>MAEKPKLHYFNARGRMESTRWLLAAAGVEFEEKFIKSAEDLDKLRNDGYLMFQQVPMVEIDGMKLVQTRAILNYIASKYNLYGKDIKERALIDMYIEGIADLGEMILLLPVCPPEEKDAKLALIKEKIKNRYFPAFEKVLHHHGQDYLVGNKLSRADIHLVELLYYVEELDSSLISSFPLLKALKTRISNLPTVKKFLQPGSPRKPPMDEKSLEEAR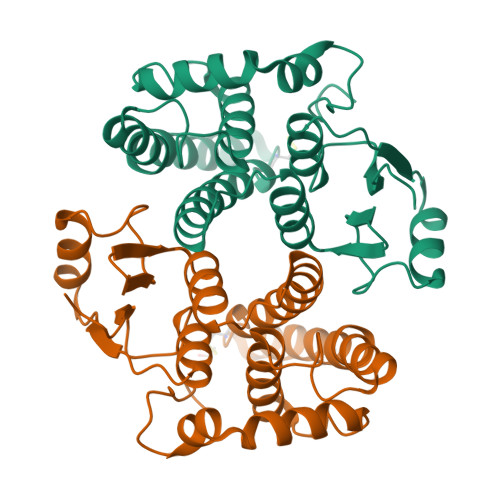KIFRF[4x]>MAEYTLPDLDWDYGALEPHISGQINELHHSKHHATYVKGANDAVAKLEEARAKEDHSAILLNEKNLAFNLAGHVNHTIWWKNLSPNGGDKPTGELAAAIADAFGSFDKFRAQFHAAATTVQGSGWAALGWDTLGNKLLIFQVYDEQTNFPLGIVPLLLLDMWEHAFYLQYKNVKVDFAKAFWN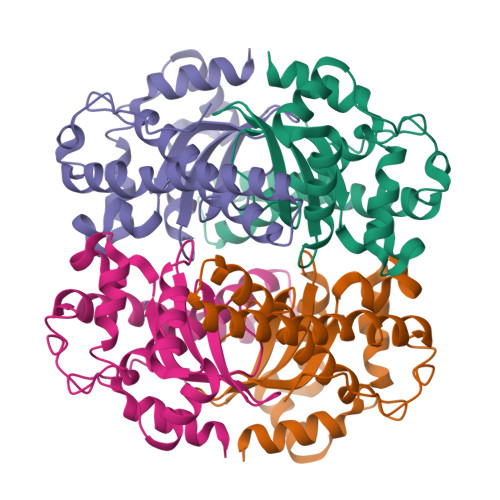VVNWADVQSRYAAATSQTKGLIFG[4x]>[2x]MDHHHHHHENLYFQMEPEESMMGMKETVSN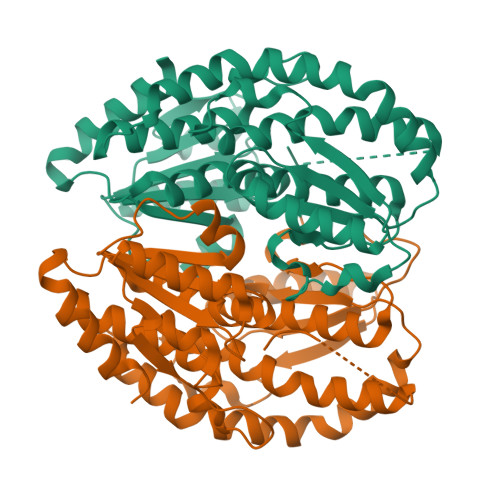IVTSQAEKGGVKHVYYVACGGSYAAFYPAKAFLEKEAKALTVGLYNSGEFINNPPVALGENAVVVVASHKGNTPETIKAAEIARQHGAPVIGLTWIMDSPLVAHCDYVETYTFGDGKDIAGEKTMKGLLSAVELLQQTEGYAHYDDFQDGVSKINRIVWRACEQVAERAQAFAQEYKDDKVIYTVASGAGYGAAYLQSICIFMEMQWIHSACIHSGEFFHGAFEITDANTPFFFQFSEGNTRAVDERALNFLKKYGRRIEVVDAAALGLSTIKTTVIDYFNHSLFNNVYPVYNRALAEARQHPLTTRRYMWKVEY> GSKTISESELSASATELLQDYMLTLRTKLSSQEIQQFAALLHEYRNGASIHEFCINLRQLYGDSRKFLLLGLRPFIPEKDSQHFENFLETIGVKDGRG;> GSMDEQEALNSIMNDLVALQMNRRHRMPGYETMKNKDTGHSNRQSDVRIKFEHNGERRIIAFSRPVKYEDVEHKVTTVFGQPLDLHYMNNELSILLKNQD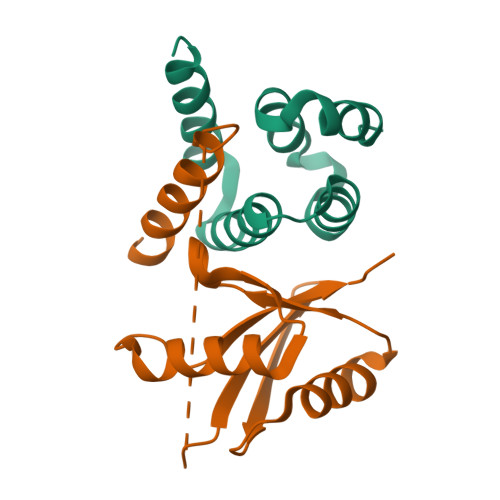DLDKAIDILDRSSSMKSLRILLLSQD>MMSDQENENEHAKAFLGLAKCEEEVDAIEREVELYRLNKMKPVYEKRDAYIDEIAEFWKIVLSQHVSFANYIRASDFKYIDTIDKIKVEWLALESEMYDTRDFSITFHFHGIEGDFKEQQVTKVFQIKKGKD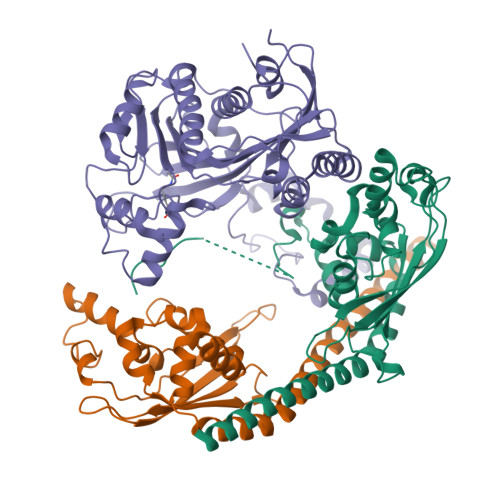DQEDGILTSEPVPIEWPQSYDSINPDLIKDKRSPEGKKKYRQGMKTIFGWFRWTGLKPGKEFPHGDSLASLFSEEIYPFCVKYYAEAQRDLEDEEGESGLSADGDSEDDDGSLGEVDLPLSDEEPSSKKRKV[2x];> GMDPNSMSLNDFLSSVLPVSEQFEYLSLQSIPLETHAVVTPNKDDKRVPKSTIKTQHFFSLFHQGKVFFSLEVYVYVTLWDEADAERLIFVSKADTNGYCNTRVSVRDITKIILEFILSIDPNYYLQKVKPAIRSYKKISPELISAASTPARTLRILARRLKQSGSTVLKEIESPRFQQDLYLSFTCPREILTKICLFTRPASQYLFPDSSKNSKKHILNGEELMKWWGFILDRLLIECFQNDTQAKLRIPGEDPARVRSYLRGMKYPLWQVGDIFTSKENSLAVYNIPLFPDDPKARFIHQLAEEDRLLKVSLSSFWIELQERQEFKLSVTSSVMGISGYSLATPSLFPSSADVIVPKSRKQFRAIKKYITGEEYDTEEGAIEAFTNIRDFLLLRMATNLQSLTGKREHRERNQPVPASNINTLAITMLKPRKKAKALPKT> MASSSHNPVILLKRILSLTESSP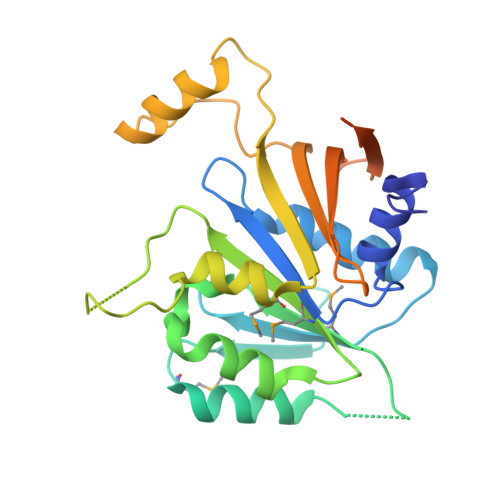FILCLDSIAQTSYKLIQEFVHQSKSKGNEYPIVYISFETVNKPSYCTQFIDATQMDFVHLVKQIISYLPAATATQAKKHMVIIDSLNYISTEYITRFLSEIASPHCTMVATYHKDIKDENRTVIPDWNNNYPDKLTLLQFMATTIVDIDVVLTGTLDTEEVSELLNEFRIPRGLNNDIFQLRLVNKRKSGRSLEYDFIVNSNTHEYELLSTTKQEEESSSNGLETPEMLQGLTTFNLGTSNKQKLAK> GSHMAFKKPLSVFKGPLLHISPAEELYFGSTESGEKKTLIVLTNVTKNIVAFK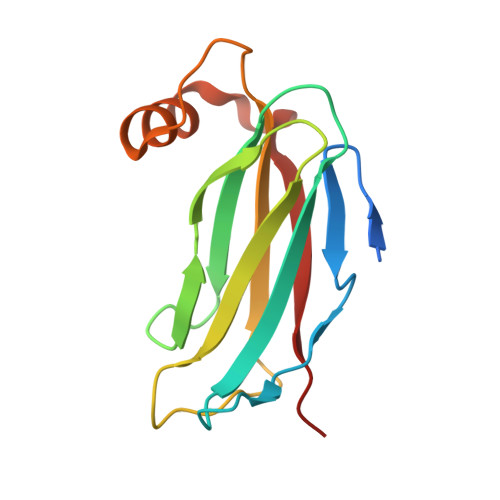VRTTAPEKYRVKPSNSSCDPGASVDIVVSPHGGLTVSAQDRFLIMAAEMEQSSGTGPAELTQFWKEVPRNKVMEHRLRCHTV> GSALSE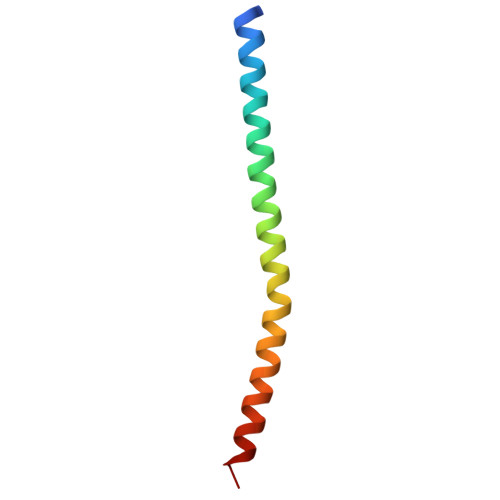IETRHSEIIKLENSIRELHDMFMDMAMLVESQGEMIDRIEYNVEHAVDYVERAVSD>[2x]MKKIPLSKYLEEHGTQSALAAALGVNQSAISQMVRAGRSIEITLYEDG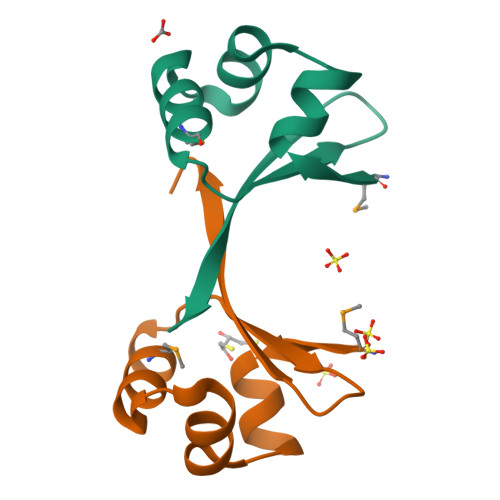RVEANEIRPIPARPKRTAA>GPLGSMVSGVNVSDECIYEFNRLKVKHLNKYIIYKIENLEKIVVDVLEHDMELTSLDNIIMRIKNNLKNTECRYIIADMPIPTPEGVLRDRIYFIFWSPGLSKPKEKMLYAASKESLVRKINGIFKSLEI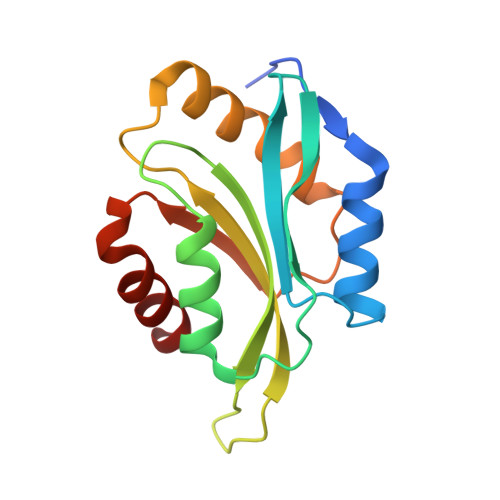TCDINEFEEELKAIILNT[2x]>[2x]MAPKKVLLALTSYNDVFYSDGMKTGVFVVEALHPFNTFRKEGFEVDFVSETGKFGWDEHSLAKDFLNGQDETDFKNKDSDFNKTLAKIKT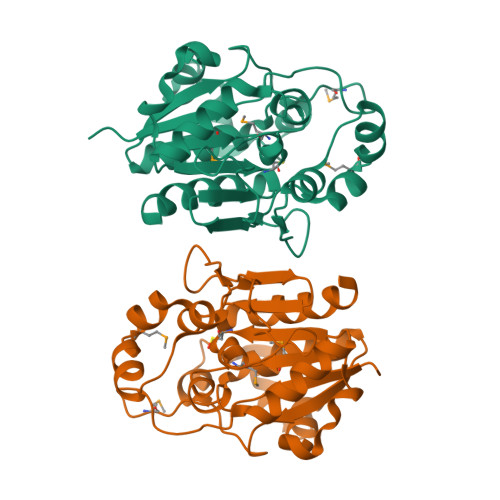PKEVNADDYQIFMASAGHGTLFDYPKAKDLQDIASEIYANGGVVAAVCHGPAMFDGLTDKKTGRPLIEGKSITGFTDVGETIMGVDSILKAKNLATVEDVAKKYGAKYLAPVGPWDDYSITDGRLVTGVNPASAHSTAVRSIDALKN> VDRLQSEPE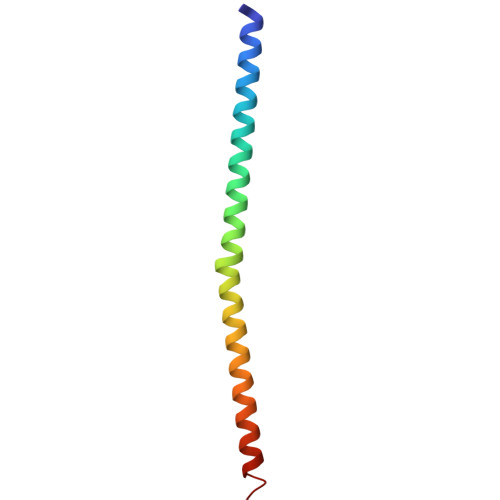SIRKWREEQTERLEALDANSRKQEAEWKEKAIKELDEWYARQDEQLQKTKANNRVADEAFY3,5-dimethyl-4-(4-pyridin-4-yl-1~{H}-pyrazol-3-yl)-1,2-oxazole | C13 H12 N4 O | 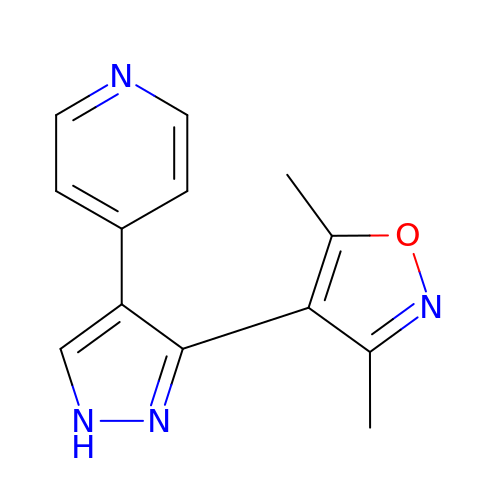JYTPHNOPQGAILG-UHFFFAOYSA-N> EETVTCLQMTVYHPGQLQCGIFQSISFNREKLPSSEVVKFGRNSNICHYTFQDKQ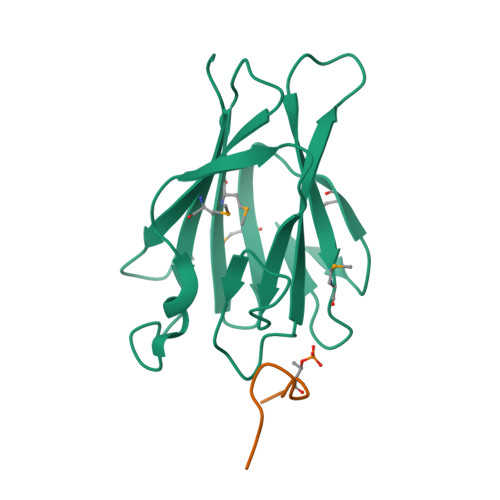VSRVQFSLQLFKKFNSSVLSFEIKNMSKKTNLIVDSRELGYLNKMDLPYRCMVRFGEYQFLMEKEDGESLEFFETQFILSPRSLLQ;> MTSFEDADTEET>MAAAAELSLLEKSLGLSKGNKYSAQGERQIPVLQTNNGPSLMGLTTIAAHLVKQANKEYLLGSTAEEKAMV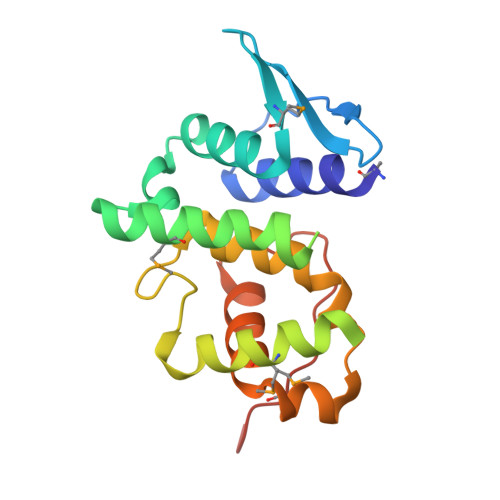QQWLEYRVTQVDGHSSKNDIHTLLMDLNSYLEDKVYLTGYNFTLADILLYYGLHRFIVDLTVQEKEKYLNVSRWFCHIQHYPGIRQHLSSVVFIKNRLYTNSH[2x]> MASSINPWILTGFADAEGSFILDIRNRNNESNRYRTSLRFQITLHNKDKSILENIQSTWKVGKITNSSDRAVMLRVTRFEDLKVIIDHFEKYPLITQKLGDYKLFKQAFSVMENKEHLKENGIKELVRIKAKMNWGLNDELKKAFPENISKERPLINKNIPNFKWLAGFTAGEGHFGVNLKKVKGTAK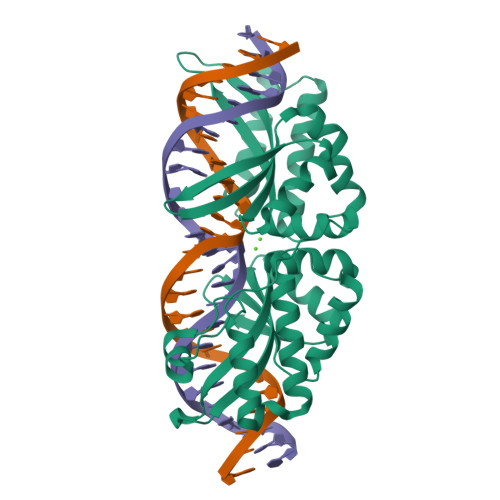VYVGLRFAISQHIRDKNLMNSLITYLGCGSIREKNKSEFRWLEFEVTKFSDINDKIIPVFQENTLIGVKLEDFEDWCKVAKLIEEKKHLTESGLDEIKKIKLNMNKGRVFS>GWVIGVDPDIGGAIAVLSPDGSSQVFDNPFVHIVVSEVIRKRLDTKSIIQLLRGLDAPPGTTAYIEKSSPFPTDGKQGWWSTGFSYGLWIASLVASGFSVVPIASQTWKAYFGLMRSETPADDSRQAASILFPDKDQSLKLKKHHGRAEALLLAAYGKGLVLP[2x]

Holliday junction resolution is a crucial process in homologous recombination and DNA double-strand break repair. Holliday junction (HJ) is a four-way structured DNA intermediate formed during the homologous recombination. Canonical HJ resolvases introduce two symmetrical nicks across the junction center by functioning as homodimers, and exhibit strong structure- and sequence-specificities in HJ cleavage. The RNase H-like enzymes, including RuvC and MOC1, typically feature three or more conserved carboxylates, known as the DDE motif, in their active sites.

To capture this transient metal ion, we mutated a critical residue K229, in vicinity of scissile phosphate. K229 is conserved across the RNase H superfamily that includes RuvC. We next crystallized MOC1K229A in complex with nHJ. Crystals were soaked into Mn2+ containing solution over various durations prior to X-ray data collection. Following incubation the crystals with Mn2+ for about 180 s, we were able to detect the occupancy of metal ions at both A and B sites, as revealed by the anomalous difference map.> SHMDYLFKLLLIGDSGVGKTCVLFRFSEDAFNSTFISTIGIDFKIRTIELDGKRIKLQIWDTAGQERFRTIT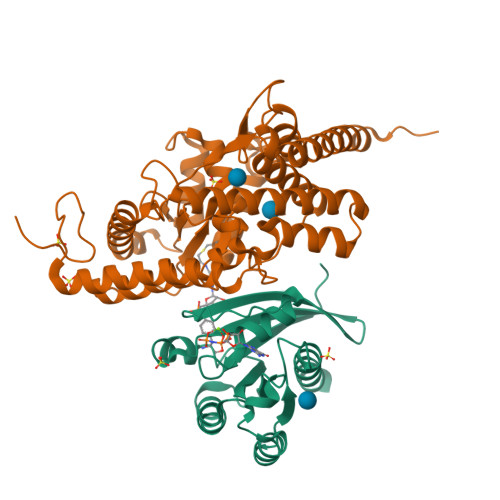TAYYRGAMGIMLVYDITNEKSFDNIRNWIRNIEEHASADVEKMILGNKCDVNDKRQVSKERGEKLALDYGIKFMETSAKANINVENAFFTLARDIKAKMDKK;> GHMFGSLYSDERDKPLLSPTAQKKFEEYQNKLANLSKIIRENEGNEVSPWQEWENGLRQIYKEMIYDAFDALGVEMPKDMEVHFAGSLAKAQATEYSDLDAFVIVKNDEDIKKVKPVFDALNNLCQRIFTASNQIYPDPIGINPSRLIGTPDDLFGMLKDGMVADVEATAMSILTSKPVLPRYECGEELRDKIKQEPSFSNMVSAKKFYNKAIKDFTAPKEGAEVVSVKTHIMRPIDFMLMGLREEFNLYSEDGAHLSAPGTIRLLREKNLLPEEQIARIESVYNQAMSKRFELHAEHKKEHDEMPYSDAKAMLDEVAKIRELGVQRVTRIENLENAKKL> IVGGQECKDGECPWQALLINEENEGFCGGTILSEFYILTAAHCLYQAKRFKVRVGDRNTEQEEGGEAVHEVEVVIKHNRFTKETYDFDIAVLRLKTPITFRMNVAPACLPERDWAESTLMTQKTGIVSGFGRTHEKGRQSTRLKMLEVPYVDRNSCKLSSSFIITQNMFCAGYDTKQEDA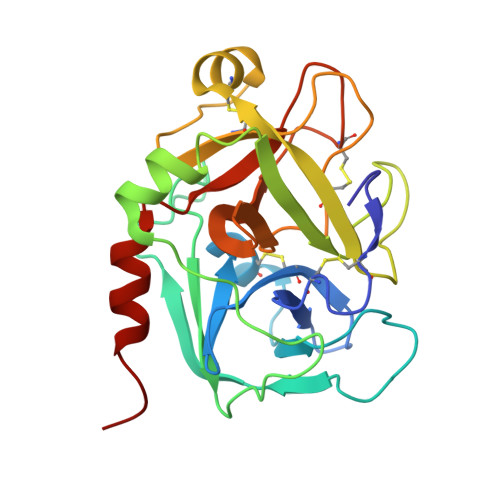CQGDSGGPHVTRFKDTYFVTGIVSWGEGCARKGKYGIYTKVTAFLKWIDRSMKTRGLP>MRGSHHHHHHGRSRSLNPLSTPQFDSTDETPASYNLAVRRAAPAVVNVYNRGLNTNSHNQLEIRTLGSGVIMDQRGYIITNKHVINDADQIIVALQDGRVFEALLVGSDSLTDLAVLKINATGGLPTIPINARRVPHIGDVVLAIGNPYNLGQTITQGIISATGRIGLNPTGRQNFLQTDASINHGNSGGALVNSLG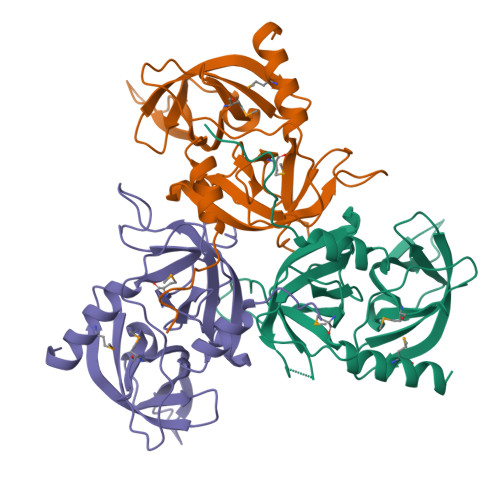ELMGINTLSFDKSNDGETPEGIGFAIPFQLATKIMDKLIRDGRVIR[9x]>TGGGGT[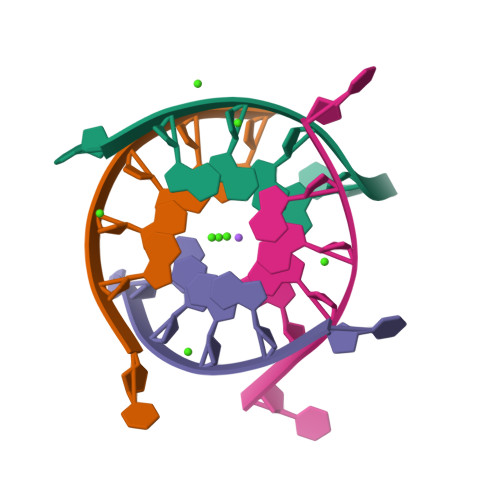8x]>[2x]AVSLDRTRAVFDGSEKSMTLDISNDNKQLPYLAQAWIENENQEKIITGPVIATPPVQRLEPGAKSMVRLSTTPDISKLPQDRESLFYFNLREIPPRSEKANVLQIALQTKIKLFYRPAAIKTRPNEVWQDQLILNKVSGGYRIENPTPYYVTVIGLGGSEKQAEEGEFETVMLSPRSEQTVKSANYNTPYLSYINDYGGRPVLSFICNG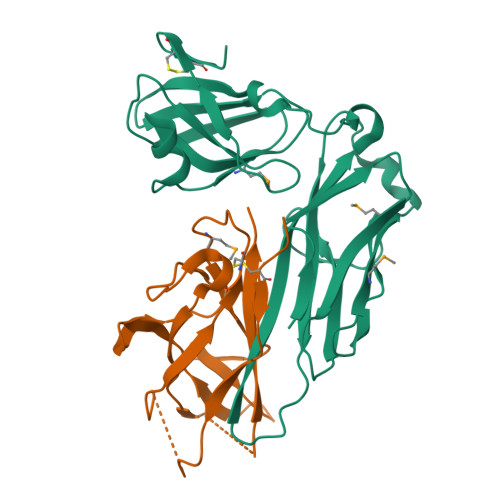SRCSVKKEKHHHHHH;>VPACTVSNTTVDWQDVEIQTLSQNGNHEKEFTVNMRCPYNLGTMKVTITATNTYNNAILVQNTSNTSSDGLLVYLYNSNAGNIGTAITLGTPFTPGKITGNNADKTISLHAKLGYKGNMQNLIAGPFSATATLVASYS[2x]(3s,5s,7s)-N-{7-[(3-O-carbamoyl-6-deoxy-5-methyl-4-O-methyl-beta-D-gulopyranosyl)oxy]-4-hydroxy-8-methyl-2-oxo-2H-1-benzopyran-3-yl}tricyclo[3.3.1.1~3,7~]decane-1-carboxamide | C30 H38 N2 O10 | 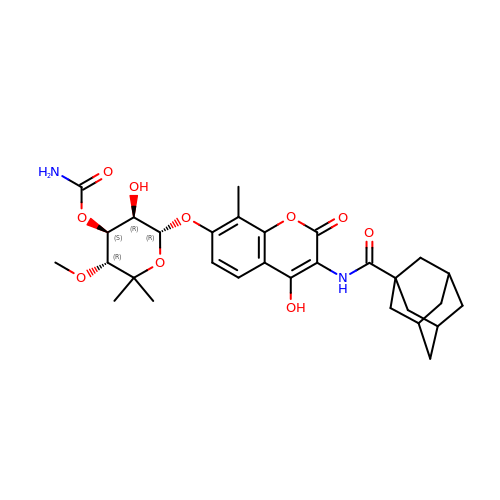SFCPIJFPMNEBLW-GGTPUZHSSA-N>MPNIKIFSGSSHQDLSQKIADRLGLELGKVVTKKFSNQE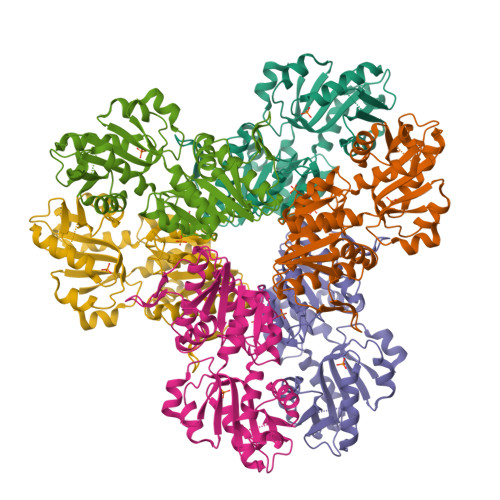TCVEIGESVRGEDVYIVQSGCGEINDNLMELLIMINACKIASASRVTAVIPCFPYARQDKKDKSRAPISAKLVANMLSVAGADHIITMDLHASQIQGFFDIPVDNLYAEPAVLKWIRENISEWRNCTIVSPDAGGAKRVTSIADRLNVDFALIHKERKKANEVDRMVLVGDVKDRVAILVDDMADTCGTICHAADKLLSAGATRVYAILTHGIFSGPAISRINNACFEAVVVTNTIPQEDKMKHCSKIQVIDISMILAEAIRRTHNGESVSYLFSHVPL[6x]>[2x]MGSDKIHHHHHHVLSKRDAILKAAVEVFGKKGYDRATTDEIAEKAGVAKGL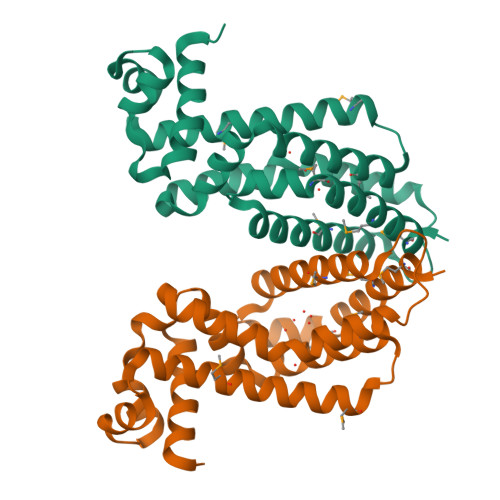IFHYFKNKEELYYQAYMSVTEKLQKEFENFLMKNRNRDIFDFMERWIEKKLEYSASHPEEADFLITLVSVDEGLRKRILLDLEKSQRVFFDFVREKLKDLDLAEDVTEEIALKFLMWFFSGFEEVYLRTYQGKPELLKRDMNTLVEEVKVMLRILKKGMTK>MAEPQPASSGLTDETAFSCCSDPDPSTKDFLLQQTMLRIKDPKKSLDFYTRVLGLTLLQKLDFPAMKFSLYFLAYEDKNDIPKDKSEKTAWTFSRKATLELTHNWGTEDDETQSYHNGNSDPRGFGHIGIAVPDVYSACKRFEELGVKFVKKPDDGKMK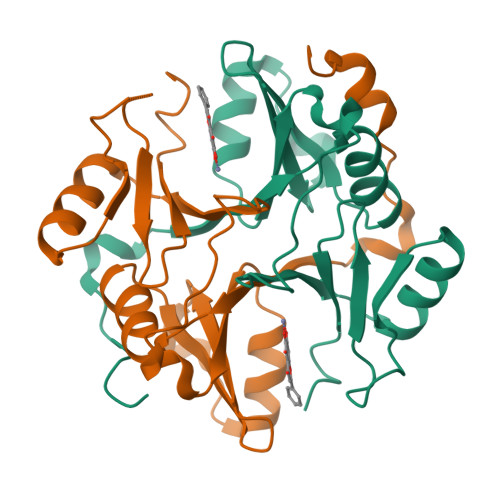GLAFIQDPDGYWIEILNPNKIATII[2x]In this study, we report the crystal structures of three forms of Tk-PTP, which showed that this protein forms a canonical DUSP fold and that it undergoes an atypical temperature-dependent conformational change between two forms. Structural and biochemical analyses revealed that this structural alteration requires the presence of the GG motif in the P-loop, and that Tk-PTP has dual amino acids, Asp63 and Glu132, both functioning as the general acid/base residues. PTP proteins commonly share a highly conserved active site motif called the PTP signature motif, which is also present in Tk-PTP as HC93MGGLGR99. This motif, constituting the phosphate binding loop (or simply called P-loop), contains the catalytic cysteine residue (Cys93) that functions as a nucleophile for dephosphorylation and the conserved arginine residue (Arg99) that anchors the phosphate group of the substrate during the enzyme reaction.

The recombinant Tk-PTP protein expressed at 25°C in Escherichia coli was purified at room temperature using a Ni–NTA column and size-exclusion chromatography, which was subsequently subjected to crystallization trials at 18°C. Triangular prism-shaped crystals were obtained, which were used for determination of the crystal structure of Tk-PTP to a resolution of 1.7 Å, referred to as Tk-PTP(form I) in this manuscript. The asymmetric unit of the crystal (space group P212121) contains one molecule of Tk-PTP(form I), in which a central β-sheet constituted by five β-strands [β1(Lys6−Asp9), β2(Val12−Ser15), β3(Ala32−Val34), β4(Glu55−His58), and β5(Lys88−His92)] is sandwiched by four helices [α2(Val69−Glu85), α3(Gly98−Arg112), α4(Leu116−Lys126), and α5(Gln134−Arg146)] on one side, and by two helices [α1(Glu22−Asp29) and α+(Leu46−Arg52)] on the other. The overall structure indicated that Tk-PTP(form I) adopts the typical DUSP fold, composed of a core region (β1–β5 and α2–α5) and mid-domain variations (α1 and α+). Similarly, Tk-PTP(form I) adopts a distorted P-loop conformation in which the backbone amides of Gly95−Gly98 are oriented away from the active site pocket (left top). Structural alignment between the P-loops of Tk-PTP(form I) and DUSP3 bound to 2-(N-morpholino)-ethanesulfonic acid (commonly called MES) shows that the main chain backbone of the residues Met94−Leu97 of Tk-PTP(form I) are arranged differently from that of the corresponding residues of DUSP3. Furthermore, steric hindrance occurs between Tk-PTP(form I) and the DUSP3-bound phosphotyrosine-mimicking molecule in the superposed model, demonstrating that the active site motif of Tk-PTP(form I) is not suitable to accommodate a phosphotyrosine moiety; therefore, Tk-PTP(form I) should have limited phosphatase activity.

> MWPSAKFIDGRVAFSRMPAERELDEVARDFDAVVVLVEDYELPYSLDEWEKRGVEVLHGPIPDFTAPSVEQLLEILRWIEERVREGKKVLIHCMGGLGRSGTVGVAWLMYSRGLSLREALMEVRRKRPGAVETQEQMEVLKELEERI> GSGAMQNSQEMAITTLSLPKGGGAINGMGESVGQAGPDGMVTFSIPLPFSAGRGVAPALSLSYSSGAGNGPFGMGWQCSAMSISRRTQKGVPQYNEDDEFLSPSGEVMAIALNDSGFEDVRTANRLQGIPLPFSYKVTRY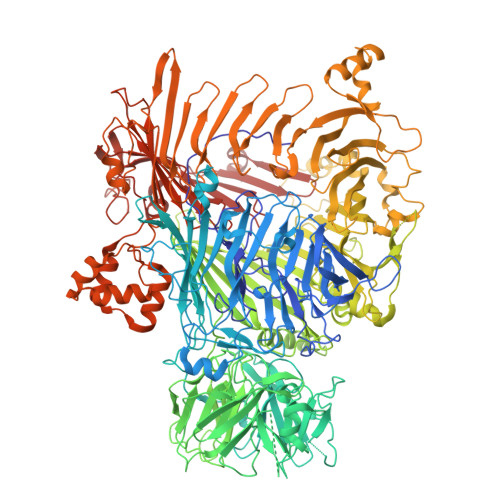QPRLIQDFIKIEYWQPVKQTDGTPFWIIYSPDGQTHILGKNSHSRVANAENPSQIASWLLEETVTPTGEHIYYQYSGENQVNCTDAEIALHPQDSAQRYLARIDYGNISPQASLFVLDEELPNLTQWLFHLVFDYGERDISINKIPTFEGGTTGWLARPDMFSRYDFGIEIRNRRLCHQVLGFHRLEALNDRDVTDEIPVLVNRLTLDYDLNNSVSTLVAVRQVAYETDGSPITQPPLEFDYQRFDTGSIPGWQEMPQLEAFNGYQPYQMIDLYGEGTPGILYQETPGAWWYKSPQRQIGGDSNAVTYGAMKALPKIPRLQEGATLMDINGDGRLDWVITSAGVRGFHSIHSTGEWTHFTPLNTLPTEYFHPKAQLADLVGAGLSDLVLIGPKSVRLYANQQGNWAPAQDVTQAENVSLPVIGIDSRQLVAFADMLGSGQQHLVEITADSVKCWPNMGHGRFGQPLTLEGFSQPQTSFNPDRVFLADIDGSGTNDIIYAHSECLEIYLNESGNRFSKPISLLLPDGVNFDNTCQLQAADIQGLGIASLVMTVPHMSPTHWRCDLALNKPWLLNVMNNNRGAETCLFYRSSAQFWLDEKQLVEAAGQQPECHLPFPMHLHWRSEIFDEITGNRLTQEQEYAHGSWDGQEREFRGFGRLIQRDTDGFAQGTVDIPTHPSRTVSWFATGIPEIDTTLSAEFWRGDDQAFSPFSPRFTRWENDSEAGSDVAFIPSEHDAFWLNRAMKGQLLRSELYGDDGTPEAEIPYSVTEMRHQVRALPTTDATVPSAWCSTIETRSYQYQRVAADPQCSQQVVIKADRYGSPLLSVAINYPRRKKPEKSPYPDDLPETLFDSSYDTQQQQLHLTKQQQNYFHLTNDDNWLLGLPKEQRNDGYQYDQERAPANGFTLETLIASNSLIGSNQPFTYLGQSRVAYQGGVDEQPSLQALVAYGETAILDEKTLQAFVGVLDSKTRDELLFSAGYQLAPRLFRVESEPDVWVARQGYSEFGDYSQFWRPLSQRSTLLTGKTTLKWDKHYCVVIETQDAAQLVTQARYDYRFLTPYSLTDANDNQHYVVLNPFGEVIASRFWGTEAGKDAGYSTPQAKPFVVPATIEAALALSPGIPVAHCAIFEPESWMQKLTQHDVSERMADNGTLWNALLQARFVTEDGYVCALGRRRWMARHGLSVLMLTLLAEIPRTPPHSLTITTDRYDSDDQQQLRQRILFSDGFGRLLQSAQRVEAGESWQRSEDSSLVVNVSGTPALVVTDNRWAVSGRTEYDGKGQGIRVYQPYFLDDWRYLSDDSARTDLFADTHIYDPLGREYQVITAKGYRRERQYTPWFVVNQDENDTAANLAI1-(3-CARBAMIMIDOYL-BENZYL)-1H-INDOLE-2-CARBOXYLIC ACID 3-CARBAMIMIDOYL-BENZYLESTER | C25 H23 N5 O2 | 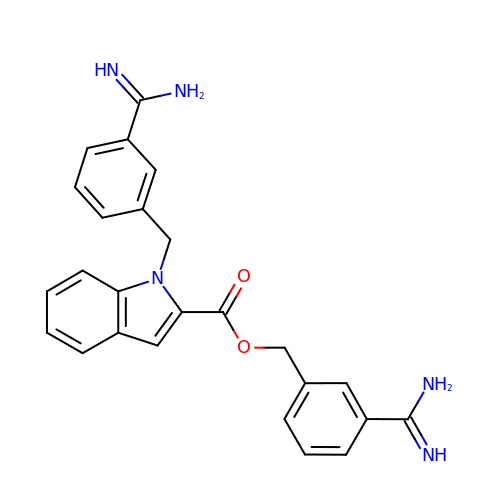ZJZBBFMRHRUCQD-UHFFFAOYSA-N> SRCTHLENRDFVTGTQGTTRVTLVLELGGCVTITAEGKPSMDVWLDAIYQESPAKTREYCLHAKLSETKVAARCPTMGPAVLTEERQIGTVCKRDQSDRGWGNHCGLFGKGSIVACVKAACEAKKKATGYVYDANKIVYTVKVEPHTGDYVAANETHKGRKTATFTVSSEKTILTLGEYG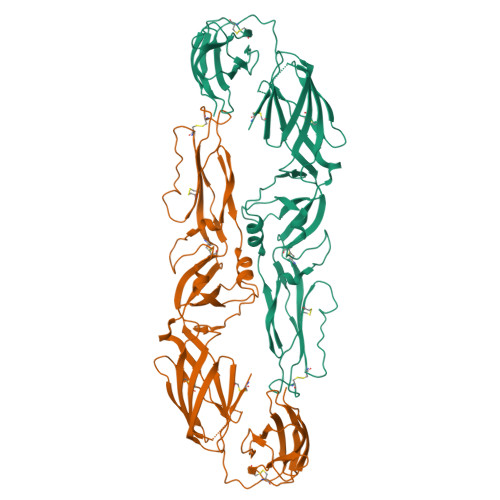DVSLLCRVASGVDLAQTIILELDKTAEHLPTAWQVHRDWFNDLALPWKHDGNPHWNNAERLVEFGAPHAVKMDVYNLGDQTGVLLRALAGVPVAHIEGNKYHLKSGHVTCEVGLEKLKMKGLTYTMCDKSKFAWKRTPTDSGHDTVVMEVTFSGSKPCRIPVRAVAHGSPDVNVAMLITPNPTIENDGGGFIEMQLPPGDNIIYVGELSHQWFQTGSSIGR>GHMSDKGKLSLQDVAELIRARACQRVVVMVGAGISTPSGIPDFRSPGSGLYSNLQQYDLPYPEAIFELPFFFHNPKPFFTLAKELYPGNYKPNVTHYFLRLLHDKGLLLRLYTQNIDGLERVSGIPASKLVEAHGTFASATCTVCQRPFPGEDIRADVMADRVPRCPVCTGVVKPDIVFFGEPLPQRFLLHVVDFPMADLLLILGTSLEVEPFASLTEAVRSSVPRLLINRDLVGPLAWHPRSRDVAQLGDVVHGVESLVELLGWTEEMRDLVQRETGKLD[6x]

Sirtuins constitute a family of NAD+-dependent enzymes that catalyse the cleavage of various acyl groups from the ∊-amino group of lysines. Sirtuins consist of a highly conserved catalytic deacylase domain of around 275 amino acids that is flanked by unstructured N- and C-termini that differ in their length and in their sequence. Of the seven members of the human sirtuin family, Sirt2 is mainly found in the cytoplasm, while Sirt3 is the main mitochondrial deacylase.

We obtained well diffracting crystals of Sirt3 in its apo form and of Sirt2 in complex with the product analogue ADP ribose (ADPR) in diverse crystallization conditions. Again, apo Sirt3 crystallized rapidly in diverse conditions, over a wide pH range and at different temperatures within days. The formation of the apo Sirt3 crystals was therefore dependent on the presence of microseeds. Sirt3 crystallized in space group P21 with six monomers in the asymmetric unit. All monomers feature the typical sirtuin-like two-domain structure with a larger Rossmann-fold domain and a smaller zinc-binding domain and adopt the ‘open’ conformation. However, they do show some differences within the asymmetric unit (r.m.s.d. ranging from 0.2 to 0.8 Å for all Cα atoms of each monomer). A similar behaviour has also been observed in the published crystal structure of human apo Sirt3. Similar to the published X-ray structure of apo Sirt3, the acyl-lysine binding site of all monomers is occupied by a PEG molecule. Using these MMS apo Sirt3 crystals, we were able to solve the X-ray structure of apo Sirt3 at a higher resolution than in the deposited X-ray structure.> VDCSEYPKPACTEEYRPLCGSDNKTYGNKCNFCNAVVESN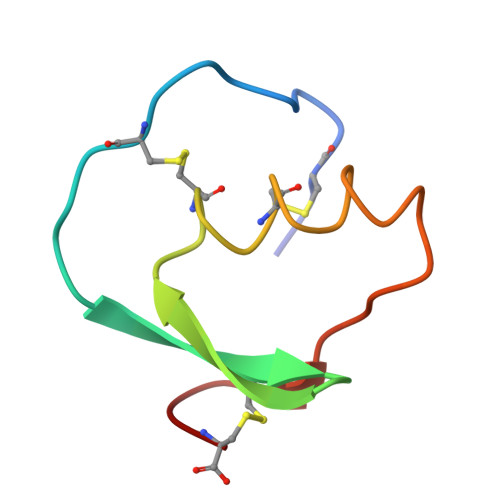GTLTLSHFGKC>[3x]MHHHHHHSSGLVPRGSMILHAQAKHGKPGLPWLVFLHGFSGDCHEWQEVGEAFADYSRLYVDLPGHGGSAAISVDGFDDVTDLLRKTLVSYNILDFWLVGYSLGGRVAMMAACQGLAGLCGVIVEGGHPGLQNAEQRAERQRSDRQWVQRFLTEPLTAVFADWYQQPVFASLNDDQRRELVALRSNNNGATLAAMLEATSLAVQPDLRANLSARTFAFYYLCGERDSKFRALAAELAADCHVIPRAGHNAHRENPAGVIASLAQILRF

Re-annotation of the activity of an earlier enzyme in the pathway, MenD, then led to the recognition that the true enzymatic activity of MenH is to covert the MenD reaction product, 2-succinyl-5-enolpyruvyl-6-hydroxy-3-cyclohexene-1-carboxylate (SEPHCHC) to 2-succinyl-6-hydroxy-2,4-cyclohexadiene-1-carboxylate (SHCHC) by a 2,5 elimination of pyruvate from the cyclohexene ring. MenH is thus correctly annotated as SHCHC synthase. EcMenH adopts a typical α/β-hydrolase fold, comprising a core β-sheet of mostly parallel strands surrounded on both sides by α-helices. As is characteristic of the α/β-hydrolases the three catalytic triad residues (Ser86, His232, Asp210) are located on loops of the core α/β–domain.

Accordingly, we report the structure of the MenH from E. coli at 2.75 Å resolution, along with the structures of two active site mutant enzymes, Arg124Ala and Tyr85Phe, both at 2.5 Å resolution. Each of the structures contains three independent molecules (A, B and C) in the asymmetric unit but EcMenH appears to be monomeric in solution on the basis of size exclusion chromatography and dynamic light scattering (results not shown). In the case of EcMenH the helical lid sits over the loops containing the active site catalytic triad residues and form part of the active site cavity. A notable feature of the active site cavity is the presence of two anions that are consistently found bound in all EcMenH structures, occupying the same sites in each. The sulfate ion forms hydrogen bonded ion pairs with both Arg90 and Arg124, which appear to be the primary determinants of binding. The chloride ion makes one charge interaction, with NH2 of Arg168, and additional interactions at distances of 2.9–3.4 Å from the OH groups of Tyr85 and Tyr148 and the side chain ND2 of Asn233. Given that the SEPHCHC substrate has three anionic groups, the carboxyl groups of the enol-pyruvate moiety, the SEPHCHC ring, and the succinyl moiety, it seems likely that the bound anions in the EcMenH crystal structure indicate key substrate interaction sites. The structure also contains candidates, the main chain NH groups from Leu87 and Phe23, for the classical oxyanion hole of the α/β hydrolases. In most chains of the native and mutant EcMenH structures there is a conserved water molecule located within a suitable distance and orientation to form hydrogen bonds with the NH groups forming this “traditional oxyanion hole”. For the native structure, for example, TS docking with no distance constraints resulted in all solutions being “succinyl-in” for chains A and C, together with the top 3 solutions for chain B. In each case the top solutions agreed to within an rms deviation of 1.5 Å.> MQVIPACNSAAIRSLCPTPESFRNMGWLSVSDAVYSEFIGELATRASNRNYSNEFGLMQPIQEFKAFIESDPVVHQEFIDMFEGIQDSPRNYQELCNMFNDIFRKAPVYGDLGPPVYMIMAKLMNTRAGFSAFTRQRLNLHFKKLFDTWGLFLSSKDSRNVLVADQFDDRHCGWLNERALSAMVKHYNGRAFDEVFLCDKNAPYYGFNSYDDFFNRRFRNRDIDRPVVGGVNNTTLISAACESLSYNVSYDVQSLDTLVFKGETYSLKHLLNNDPFTPQFEHGSILQGFLNVTAYHRWHAPVNGTIVKIINVPGTYFAQAPSTIGDPIPDNDYDPPPYLKSLVYFSNIAARQIMFIEADNKEIGLIFLVFIGMTEISTC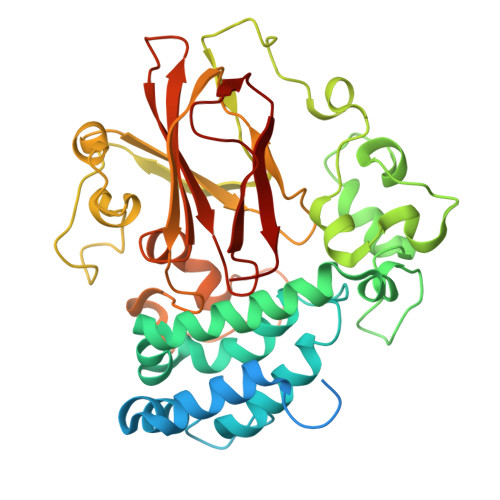EATVSEGQHVNRGDDLGMFHFGG> MHHHHHHMSSSDGKLRYDGRVAVVTGAGAGLGREYALLFAERGAKVVVNDLGGTHSG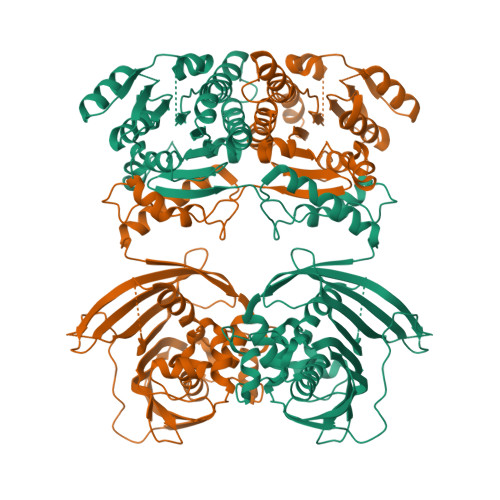DGASQRAADIVVDEIRKAGGEAVADYNSVIDGAKVIETAIKAFGRVDILVNNAGILRDRSLVKTSEQDWNLVNDVHLKGSFKCTQAAFPYMKKQNYGRIIMTSSNSGIYGNFGQVNYTAAKMGLIGLANTVAIEGARNNVLCNVIVPTAASRMTEGILPDILFNELKPKLIAPVVAYLCHESCEDNGSYIESAAGWATKLHMVRGKGAVLRPSLDDPVTIEYVKDVWSNVTDMSKAKHLGAIAEASGTLLEVLEKLKEGGGDAIEDAFEFNSKELITYALGIGASVKNAKDMRFLYENDADFAAIPTFFVLPGLLLQMSTDKLLSKALPNSQVDFSNILHGEQYLEIVDDLPTSGTLLTNGKVFDVMDKGSGAVVVTNSESFDESGRLLVRNQSTTFIVGAGKFGGKKDPIAGVVPLQPAPNRQPDATVQYTTSEDQAALYRLSGDKNPLHIDPQMALLAGFKTPILHGLCTLGFSVRAVLAQFADNNPALFKAVKVRFSGPVIPGQTLRVDLWKQGTRINFRTVVVETGKEVISGAYVDLKSSQAKLLEHHHHHH2-(4,6-dimethylpyrimidin-2-yl)sulfanyl-N-(4-phenylsulfanylphenyl)ethanamide 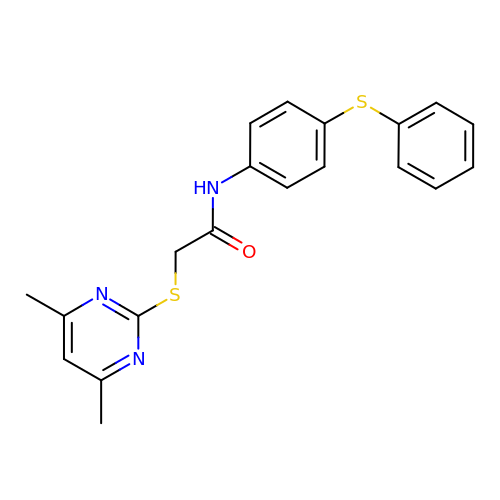| C20 H19 N3 O S2 | KOUOSAPHOUALKH-UHFFFAOYSA-N3-cyclopentyl-~{N}-(3-piperidin-1-ylphenyl)propanamide 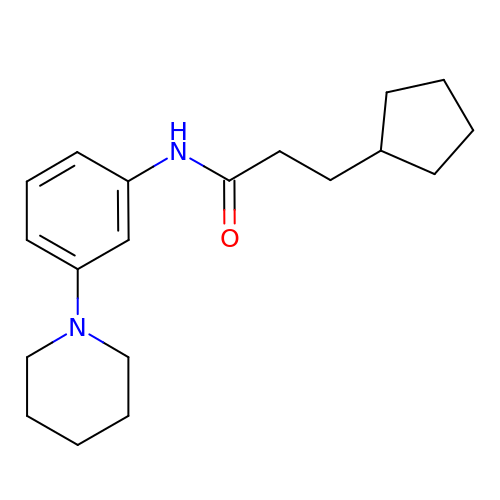| C19 H28 N2 O | ICGIQDRKVXQXTR-UHFFFAOYSA-N>MMSPRIGLTLQKIVETAAEIADANGVQEVTLASLAQTLGVRSPSLYNHVKGLQDVRKNLGIYGIKKLHNRLEEAAEDKRMDEAIHALGEAYVAFVRKHPGLYEATFLRDEEVRKAGDGIVKLCLQVLQQYGLEGENALHATRGFRSICHGFASIEQQGG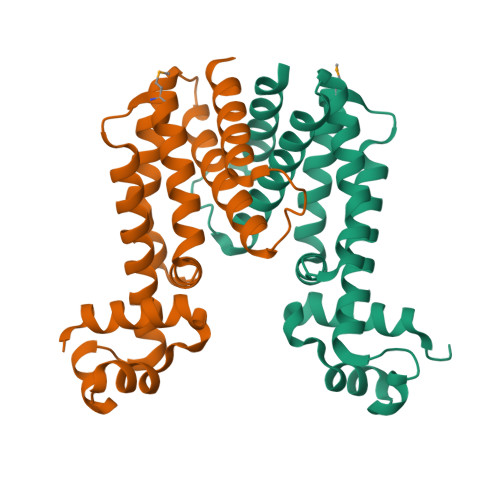FGLPLDLDISLHVLLETFIKGLRE[2x]> IVGGYTCQENSVPYQVSLNSGYHFCGGSLINDQWVVSAAHCYKSRIQVRLGEHNINVLEGNEQFVNAA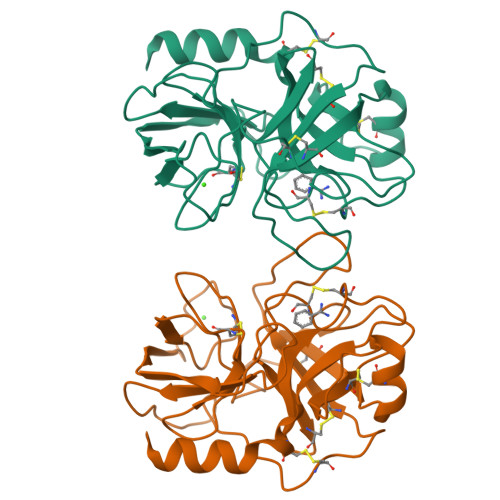KIIKHPNFDRKTLNNDIMLIKLSSPVKLNARVATVALPSSCAPAGTQCLISGWGNTLSSGVNEPDLLQCLDAPLLPQADCEASYPGKITDNMVCVGFLEGGKGSCQGDSGGPVVCNGELQGIVSWGYGCALPDNPDVYTKVCNYVDWIQDTIAAN> MLGAIAYTGNKQSLLPELKSHFPKYNRFVDLFCGGLSVSLNVNGPVLANDIQEPIIEMYKRLINVSWDDVLKVIKQYKLSKTSKEEFLKLREDYNKTRDPLLLYVLHFHGFSNMIRINDKGNFTTPFGKRTINKNSEKQYNHFKQNCDKIIFSSLHFKDVKILDGDFVYVDPPYLITVADYNKFWSEDEEKDLLNLLDSLNDRGIKFGQ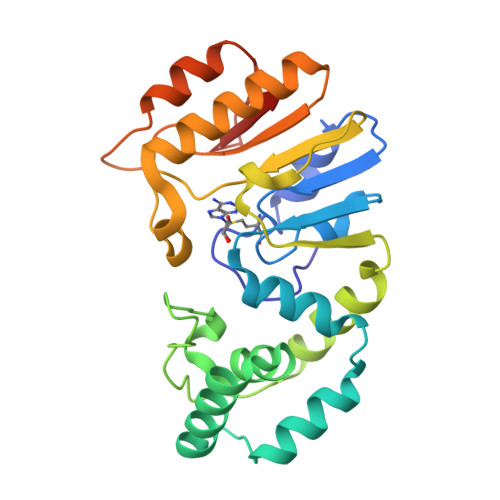SNVLEHHGKENTLLKEWSKKYNVKHLNKKYVFNIYHSKEKNGTDEVYIFN EDROPHONIUM ION | C10 H16 N O | 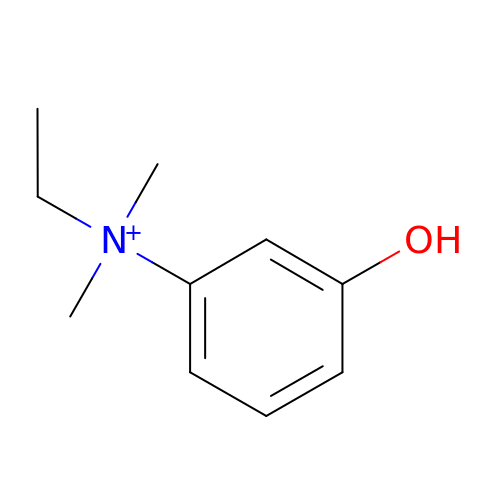VWLHWLSRQJQWRG-UHFFFAOYSA-O>MKPKKNQYQQMQGMGMGMDMQGFQPQLGPNPYPQPQGQGSQMMPMQQQMTMPMQQGQQGFGGGFPGQPQQQGGGSFQIPSGPSSSQNVPGMLPIEESYIENILRLNRGKTATIYMTFENSKEWNSKIFRGVIEAAGRDHIIISDPK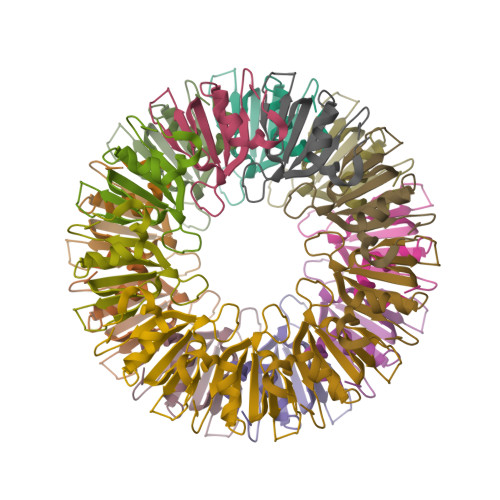TGTRYLLLTIYLDYITFDEEIAYTYPYSMSSYSPR[18x]> GPPGPPGPPGPKGHRGFSGLPGPPGP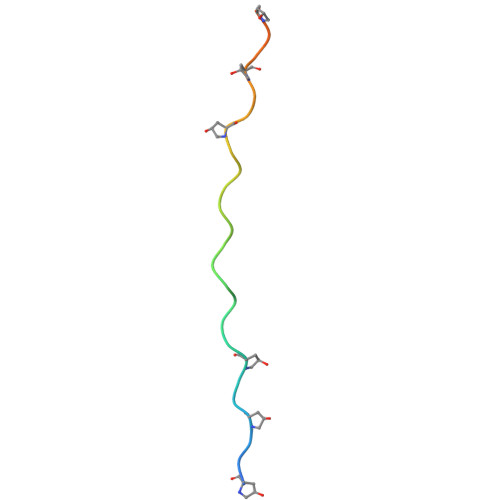PGPPGCG>[12x]MEEIIVRGGNQLNGTVRIEGAKNAVLPILAASLLAEEGITTLDNVPILSDVFTMNQVIRHLNVDVDFDEQKNQVTIDASRQLEIEAPYEYVSQMRASIVVMGPLLARNGHAKVAMPGGCAIGKRPIDLHLKGFQALGAKIIQKNGYIEAIADELIGNTIYLDFPSVGATQNIMMAAVKAKGTTIIENVAREPEIVDLANILNKMGAQVYGAGTETMRIEGVDHLHAVNHSIVQDRIEAGTFMVAAAMTQGNVLIADAISEHNRPLISKLIEMGAEIIEEEGGVRVIGPKHILPTDVKTMPHPGFPTDMQAQMTAIQLVAEGTSVVTETVFENRFQHLEEMRRMNAHVKIDGNVAIMDGNHELQGAEVYATDLRAAAALVLAGLKANGITRVRNLNYLDRGYYNFHIKLQQLGADVERVDMDQTSAEKTAQTIA

MurAA catalyzes the first committed step of peptidoglycan synthesis, transferring an enolpyruvate moiety from phosphoenolpyruvate (PEP) to UDP-N-acetylglucosamine to produce UDP-GlcNAc-enolpyruvate and inorganic phosphate. MurAA comprises two domains with the active site Cys119 located in a flexible loop (Ala114–Ile126) that is solvent exposed in the ligand-free state. We refer to the domain containing the active site loop as the “catalytic domain” (residues 21–232) and the other as the “C-terminal domain” (residues 1–20, 233–419).

In order to determine the structure of apo-MurAA, we also attempted to crystallize MurAA without added ligands or cofactors during purification and crystallization. Data were collected up to a resolution of 2.65 Å. Upon inspection of the electron density, we observed significant positive difference density near the thiol group of the active site cysteine (Cys119) and UDP-binding site at the interface of the two domains. This was surprising as we did not add any of the ligands during purification and crystallization. Based on these observations, we modeled the covalent modification at the active site cysteine as a Cys119-PEP adduct and UDP–MurNAc at the interface of two domains in E. faecium MurAA to form the dormant complex. The density for Cys-PEP adducts in all chains was well defined and unambiguous, but the electron density for UDP–MurNAc was found to be weaker and more variable across the individual copies of the asymmetric unit. The observed weaker electron density could be due to a lower occupancy of UDP–MurNAc and may be indicative of partial occupancy. Except for the position of the surface loop (Ala114–Ile126 with rmsd = 2.7 Å) the overall structures of MurAA are quite similar (C-alpha rmsd of 420 residues = 0.6 Å). In our previous study, we also identified a less common G220V substitution during the development of DAP resistance in E. faecium HOU515FΔliaR. Importantly, positions 149 and 220 are proximal to each other at the protein surface but distal to the active site consistent with a potential role in protein–protein interactions. The structures of E. faecium MurAA with FOS–UDP-GlcNAc and by serendipity UDP–MurNAc suggest that, like other members of the MurA family, the protein transitions from an open to closed conformation upon UDP-GlcNAc binding.>[4x]ACGCCGT;>ACGGCGT[4x]

We have determined the crystal structures of DNA duplexes containing -CGCCG- regions as CCG repeat motifs that comprise a non-CpG site with or without cytosine methylation. On the other hand, methylation of cytosines immediately preceding a non-guanine residue is known as non-CpG methylation. Our structural results demonstrated that cytosine methylation at a non-CpG step leads to an anti→syntransition of its complementary guanosine residue toward the (w)cWH geometry as a partial population of WC, in both drug-bound and naked mC:G base pairs. This particular geometry is specific to non-CpG methylated dinucleotide sites in B-form DNA.

To investigate the structural effects of non-CpG methylation on the DNA structure, we have determined the crystal structures of the DNA duplexes d(ACGmCCGT/ACGGCGT) (named as mC:G pairing structure)and d(ACGCCGT/ACGGCGT) (named as C:G pairing structure), which represent methylated and unmethylated states, respectively. The crystal structures of unmethylated d(ACGCCGT/ACGGCGT) (C:G pairing structure) and methylated d(ACGmCCGT/ACGGCGT) (mC:G pairing structure) were solved at resolutions of 2.35 and 2.0 Å, respectively. In these structures, oligonucleotides self-assembled into antiparallel duplexes with four independent duplexes within each asymmetric unit. The central 5-bp segment of each duplex in both the unmethylated and methylated crystal structures have B-DNA-like duplex conformations. The measured values suggest that the C4:G11 base pairs in all four unmethylated duplexes adopts a canonical Watson–Crick (WC) conformation. Because the geometry of the C4:G11 base pair in all four unmethylated duplexes were similar, C:G-NPX1 was selected as a representative of the unmethylated conformation. The mC4 and C5 bases were better aligned when compared to their unmethylated counterparts. The π–π distances between the mC4 and C5 bases in the methylated structures (3.5 Å) were also shorter than that in the unmethylated structure (3.9 Å) as shown in Figure 3D–G. These results suggest stronger stacking interactions in the methylated structures compared to the unmethylated structure.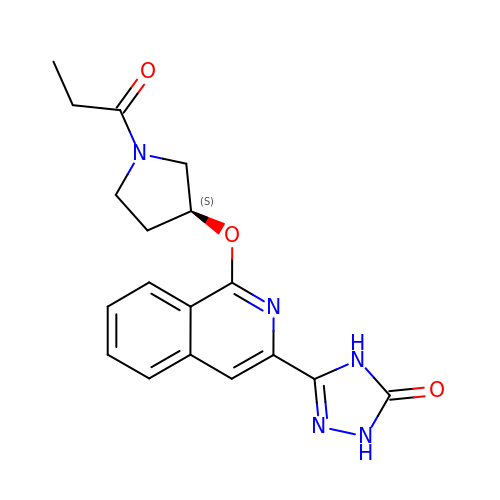5-(1-{[(3S)-1-propanoylpyrrolidin-3-yl]oxy}isoquinolin-3-yl)-2,4-dihydro-3H-1,2,4-triazol-3-one | C18 H19 N5 O3 | HTXPJYDZXSMZTC-LBPRGKRZSA-N>UCGUACGA[2x]

In order to investigate the influence of metal ions on RNA structure, six octameric RNA duplex structures were solved in the presence of different metal ions. The RNA forms a continuous helix throughout the lattice by end-to-end stacking of the asymmetric unit, as it is often seen in crystal structures of nucleic acids to maximize the energy of the base-stacking. The isomorphous structures showed the characteristics of the A-form helix. In every solved octameric structure one cation is located in the center of the major groove.

Three of the other RNA crystals were grown in the presence of calcium(II) and afterwards soaked in solutions containing either Mn2+, Cu2+, or Tb3+. In the RNA structure that was soaked in copper(II), the Ca2+ at the phosphate backbone is not replaced by Cu2+, which demonstrates the strong preference of Ca2+ for the phosphate oxygens. We found in the octameric RNA duplex a unique innersphere interaction of Cu2+ to O4 of uracil. While inner-sphere binding (e.g., to O6 of guanine) is known, to the best of our knowledge innersphere binding to uracil O4 is here observed for the first time with Cu2+, compared to other macromolecules deposited in the protein databank (PDB). Although we observe a strong anomalous signal in the central part of the major groove at the absorption edge of Cu2+, the unusual elongated bond lengths to the coordinating waters and the valence bond parameter do not suggest that only Cu2+ is located at this position. Therefore we try to quantitatively demonstrate the position of Cu2+ by integrating the area of the anomalous difference map. The occupancy of the strong anomalous scatterer Cu2+ relative to phosphorus, for which we assume 100% occupancy, was then calculated. The occupancy value for the anomalous difference map in Table 2 corresponds to the observed value from the electron density map and therefore confirms the position of Cu2+ at this site. The results indicate that the site is not fully occupied by Cu2+ and that in some structures Ca2+, instead of Cu2+, must be present. Hence, we propose a mixed state of Ca2+ with Cu2+ which was used for soaking.>METSENKSEIKILSLNGGGVRGLFTITLLAELESIIEKREKCENVKIGDYFDLITGTSIGGILALGLASGKSARELKEAFEINATKIFPLKRFKNKQWWNLLRRSIYESEPLYDAVKSMIGETIKFEDLNRRVMITSVNLSTGKPKFFKTPHNPMFTMDREIRLIDAAMATSAAPTYFKPHYIEKLENYFADGGLVANNPSYIGIREVLIDMKNDFPDAKPENIKVLNIGTLSEDYCISPETLSKNSGKGYLSLWNMGERIVLSTMTANQHLQRFMLLREFEALKIEKNYVEIDETIPNEAAAEITLDNASEGCLKALRGSGKKLAAERYTKNEELRNFFLKK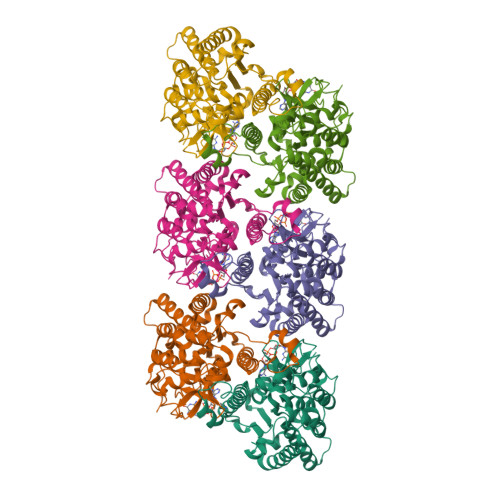AEPFVPYIESSEVTAHHHHHH[6x]8-[(6-iodo-1,3-benzodioxol-5-yl)sulfanyl]-9-[6-(triphenyl-lambda~5~-phosphanyl)hexyl]-9H-purin-6-amine 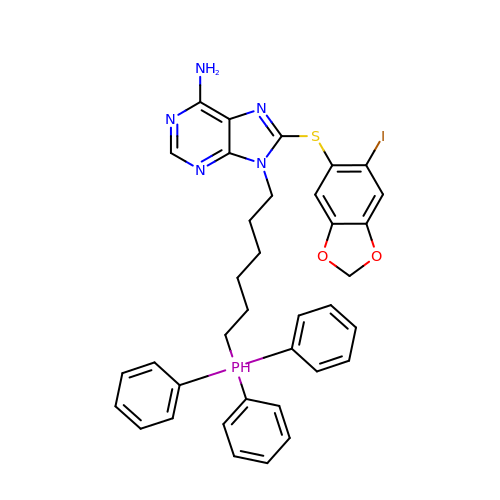| C36 H35 I N5 O2 P S | XFZHUJRJLSACIB-UHFFFAOYSA-N[(~{E})-2-[5-bromanyl-2-[(4-oxidanylidene-3,5-dihydropyrrolo[3,2-d]pyrimidin-7-yl)sulfanyl]phenyl]ethenyl]phosphonic 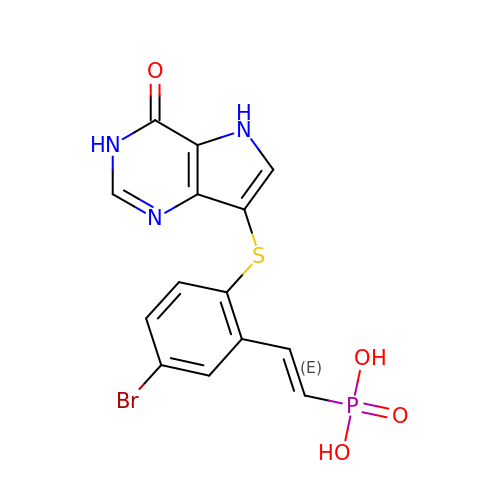acid | C14 H11 Br N3 O4 P S | MGDUXLLRMUSBMA-ONEGZZNKSA-N> DEQSGKSQTVIVGPW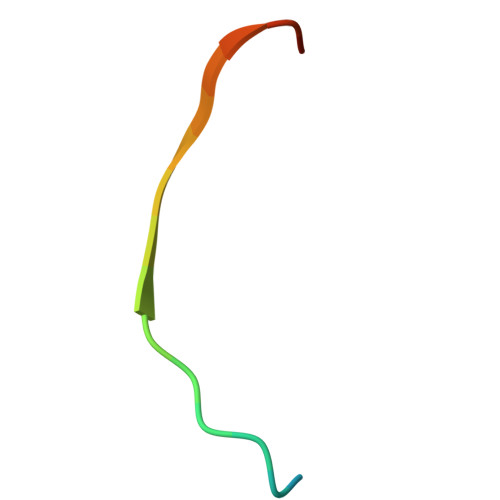GAKVS>PMFIVNTNVPRASVPEGFLSELTQQLAQATGKPAQYIAVHVVPDQLMTFSGTNDPCALCSLHSIG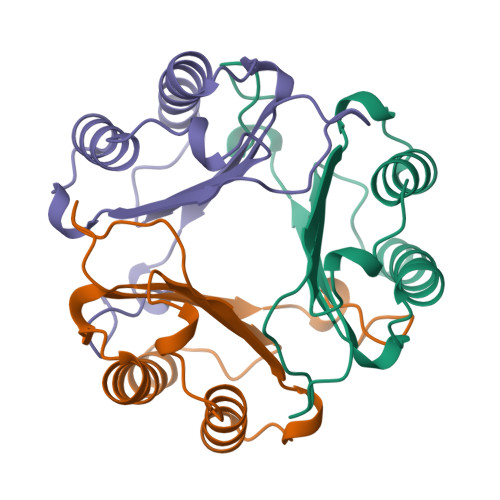KIGGAQNRNYSKLLCGLLSDRLHISPDRVFINYYDMNAANVGWNGSTFA[3x]>[2x]GSMIPYQEWHS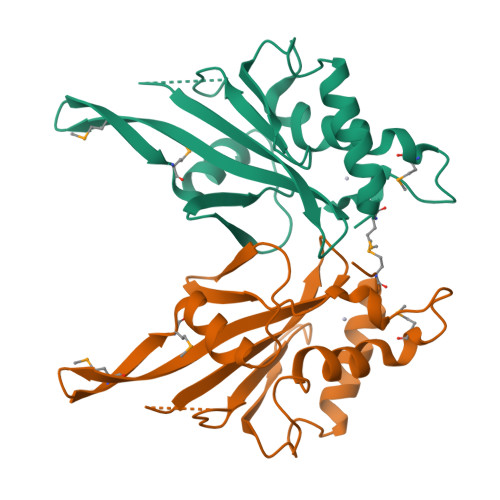QLQSLYDSQIFHNWALCQDVHLNDEKDGLLLRLIPTRQLQKNTERIENKLLNHIELYLTYSKVYNEPLLLLRIWEEKSIDGIPMTKLMLPTDIESLLDVQGKFQLGLDTIINLEGSVWYSFHPCDTSCIVGDQAEFMSTYLRRWVSIFIFSWLGYEDS>EGICRNRVTNNVKDV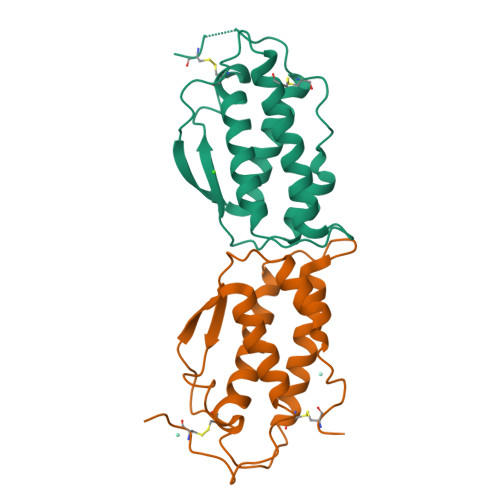TKLVANLPKDYMITLKYVPGMDVLPSHCWISEMVVQLSDSLTDLLDKFSNISEGLSNYSIIDKLVNIVDDLVECVKENSSKDLKKSFKSPEPRLFTPEEFFRIFNRSIDAFKDFVVASETSDCVVS[4x]> TQAKAKHADVPVNLYRPNAPFIGKVISNEPLVKEGGIGIVQHIKFDLTGGNLKYIEGQ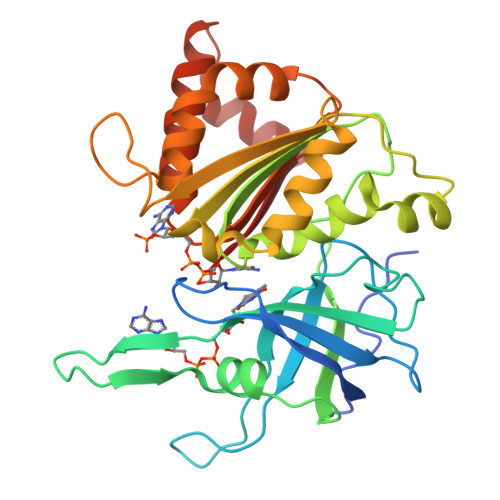SIGIIPPGVDKNGKPEKLRLYSIASTRHGDDVDDKTISLCVRQLEYKHPESGATVYGVCSTYLTHIEPGSEVKITGPVGKEMLLPDDPEANVIMLATGTGIAPMRTYLWRMFKDAERAANPEYQFKGFSWLVFGVPTTPNILYKEELEEIQQKYPDNFRLTYAISREQKNPQGGRMYIQDRVAEHADQLWQLIKNQKTHTYICGLRGMEEGIDAALSAAAAKEGVTWSDYQKDLKKAGRWHVETS>[5x]MNSTLLPTDIVGGTFWLLSMALIGASIFFLLERNRVDGR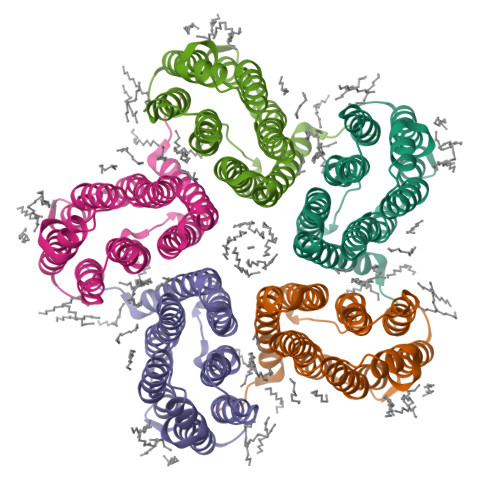WHTTMTLLGVTMLISAIFYYYVQGMWVDTGKAPIVLRYLDWILTHSMQVVMFYVILTAVTKVSSALFWRLLIGALVMVIGEFLGAAGYMSATLGFIIGVVGWLYILGEIYMGEASRCNIESGNEATHMAFNGLRLILTIGWAIYPLGYFINNLGGGVDANSLNIIYNLTDFLNKIIFGFVVYRAAMNDTQARLDEIKKLEHHHHHH>MAGLPNSSNALQQWHHLFEAEGTKRSPQAQQHLQQLLRTGLPTRKHENWKYTPLEGLINSQFVSIAGEISPQQRDALALTLDSVRLVFVDGRYVPALSDATEGSGYEVSINDDRQGLPDAIQAEVFLHLTESLAQSVTHIAVKRGQRPAKPLLLMHITQGVAGEEVNTAHYRHHLDLAEGAEATVIEHFVSLNDARHFTGARFTINVAANAHLQHIKLAFENPLSHHFAHNDLLLAEDATAFSHSFLLGGAVLRHNTSTQLNGENSTLRINSLAMPVKNEVCDTRTWLEHNKGFCNSRQLHKTIVSDKGRAVFNGLINVAQHAIKTDGQMTNNNLLMGKLAEVDTKPQLEIYADDVKCSHGATVGRIDDEQIFYLRSRGINQQDAQQMIIYAFAAELTEALRDEGLKQQVLARIGQRLPGGAR[2x];>MGSSHHHHHSSGLVPRGSHMLSIKDLHVSVEDKAILRGLSLDVHPGEVHAIMGPNGSGKSTLSATLAGREDYEVTGGTVEFKGKDLLALSPEDRAGEGIFMAFQYPVEIPGVSNQFFLQTALNAVRSYR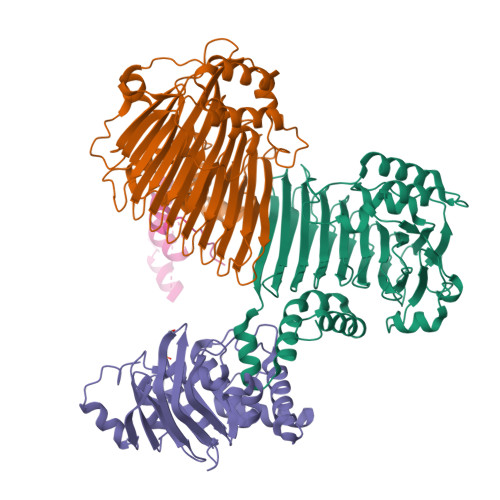GQETLDRFDFQDLMEEKIALLKMPEDLLTRSVNVGFSGGEKKRNDILQMAVLEPELCILDESDSGLDIDALKVVADGVNSLRDGKRSFIIVTHYQRILDYIKPDYVHVLYQGRIVKSGDFTLVKQLEEQGYGWLTEQQ[2x]>[2x]GPLHMVKVALAGCPNVGKTSLFNALTGTKQYVANWPGVTVEKKEGVFTYKGYTINLIDLPGTYSLGYSSIDEKIARDYLLKGDADLVILVADSVNPEQSLYLLLEILEMEKKVILAMTAIDEAKKTGMKIDRYELQKHLGIPVVFTSSVTGEGLEELKEKIVEYAQKNTILHRMILDYGEKVESEIKKVENFLRDKKLRINPRYFALKYLSGDPEFYSEGVKLGLPELSEEERIGYRLLIAKRKR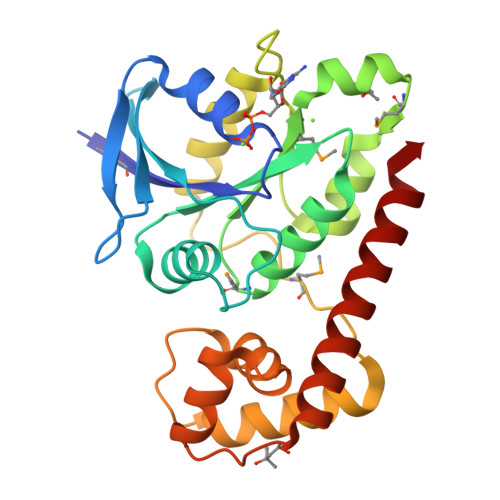EYVENVVKEAFAD> SGPINDTDANPRYKIPVEADFLFAYSTVPGYASMRNPGRGSWFVQALCSILEEHGKDLEIMQILTRVNDRVARHFESQSDDPHFHE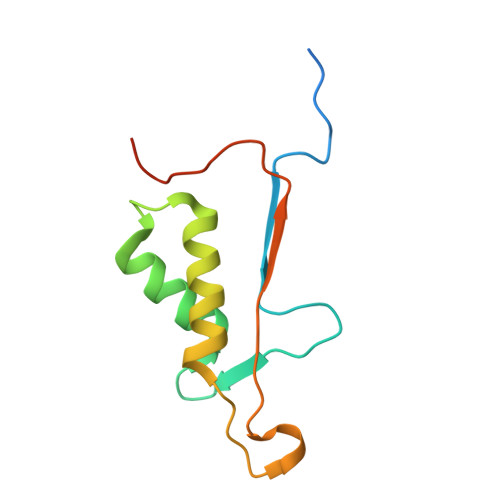KKQIPCVVSMLTKELYFSQLEHHHHHH> EDTVGRPLPHLAAAMQASGEAVYCDDIPRYENELFLRLVTSTRAHAKIKSIDVSEAQKVPGFVCFLSADDIPGSNETGLFNDETVFAKDTVTCVGHIIGAVVADTPEHAERAAHVVKVTYEDLPAIITIEDAIKNNSFYGSELKIEKGDLKKGFSEADNVVSGELYIGGQDHFYLETHCTIAIPKGEEGEMELFVSTQNAMKTQSFVAKMLGVPVNRILVRVKRMGGGFGGKETRSTLVSVAVALAAYKTGHPVRCMLDRNEDMLITGGRHPFLARYKVGFMKTGTIVALEVDHYSNAGNSRDLSHSIMERALFHMDNCYKIPNIRGTGRLCKTNLSSNTAFRGFGGPQALFIAENWMSEVAVTCGLPAEEVRWKNMYKEGDLTHFNQRLEGFSVPRCWDECLK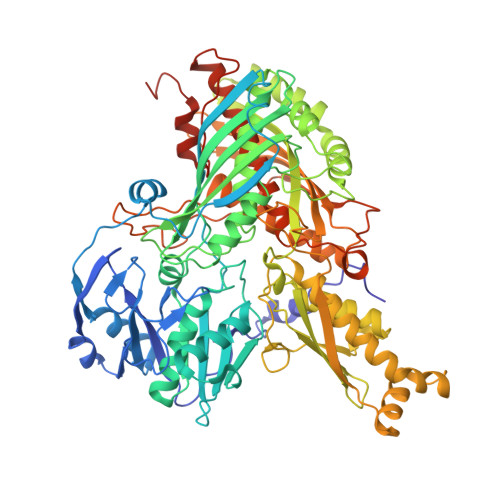SSQYYARKSEVDKFNKENCWKKRGLCIIPTKFGISFTVPFLNQAGALIHVYTDGSVLVSHGGTEMGQGLHTKMVQVASKALKIPISKIYISETSTNTVPNSSPTAASVSTDIYGQAVYEACQTILKRLEPFKKKNPDGSWEDWVMAAYQDRVSLSTTGFYRTPNLGYSFETNSGNAFHYFTYGVACSEVEIDCLTGDHKNLRTDIVMDVGSSLNPAIDIGQVEGAFVQGLGLFTLEELHYSPEGSLHTRGPSTYKIPAFGSIPTEFRVSLLRDCPNKKAIYASKAVGEPPLFLGASVFFAIKDAIRAARAQHTNNNTKELFRLDSPATPEKIRNACVDKFTTLCVTGAPGNCKPWSLRV>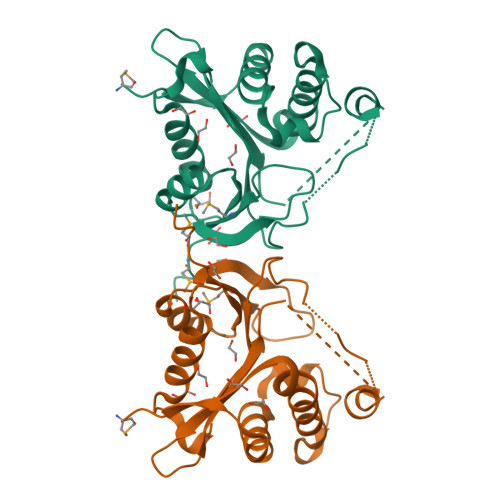 GMSPTVLPATQADFPKIVDVLVEAFANDPTFLRWIPQPDPGSAKLRALFELQIEKQYAVAGNIDVARDSEGEIVGVALWDRPDGNHSAKDQAAMLPRLVSIFGIKAAQVAWTDLSSARFHPKFPHWYLYTVATSSSARGTGVGSALLNHGIARAGDEAIYLEATSTRAAQLYNRLGFVPLGYIPSDDDGTPELAMWKPPAMPTV>GAMDPNYDKWEMERTDITMKHKLGGGQYGEVYEGVWKKYSLTVAVKTLKEDTMEVEEFLKEAAVMKEIKHPNLVQLLGVCTREPPFYIITEFMTYG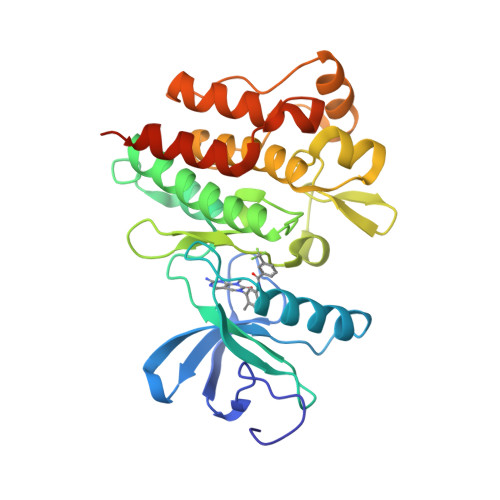NLLDYLRECNRQEVNAVVLLYMATQISSAMEYLEKKNFIHRDLAARNCLVGENHLVKVADFGLSRLMTGDTYTAHAGAKFPIKWTAPESLAYNKFSIKSDVWAFGVLLWEIATYGMSPYPGIDLSQVYELLEKDYRMERPEGCPEKVYELMRACWQWNPSDRPSFAEIHQAFETMFQESSISDEVEKELGK[2x]>QQASTLPDLAEQFAPPDVAPPLLIKLVEAIEKKGLECSTLYRTQSSSNPAELRQLLDCDTASLDLEMFDVHVLADAFKRYLLDLPNPVIPVAVSSELISLAPEVQSSEEYIQLLKKLIRSPSIPHQYWLTLQYLLKHFFKLSQTSSKNLLNARVLSELFSPLLFRFPAASSENTEHLIKIIEILIST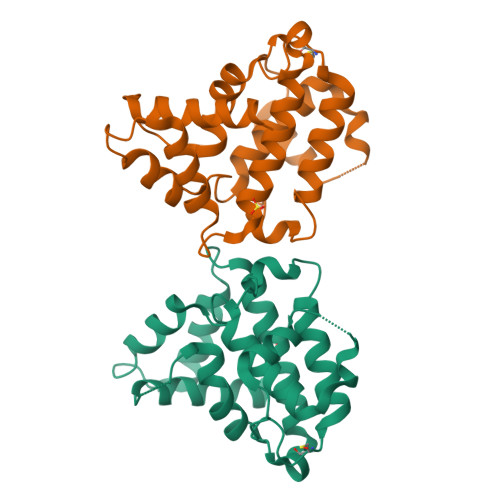KWNERQ[2x]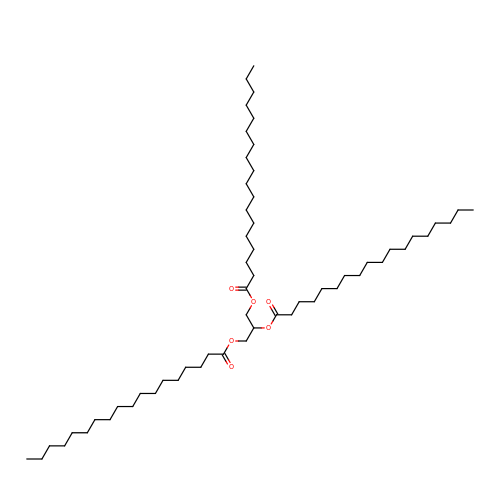TRISTEAROYLGLYCEROL | C57 H110 O6 | DCXXMTOCNZCJGO-UHFFFAOYSA-N>[4x]SNAGGRAAGTGGGGPSAPVDKEVDYAQYFCTYSFLYHQKDMLSDRVRMDAYFNAVFQNKHHFEGKTVLDVGTGSGILAIWSAQAGARKVYAVEATKMADHARALVKANNLDHIVEVIEGSVEDISLPE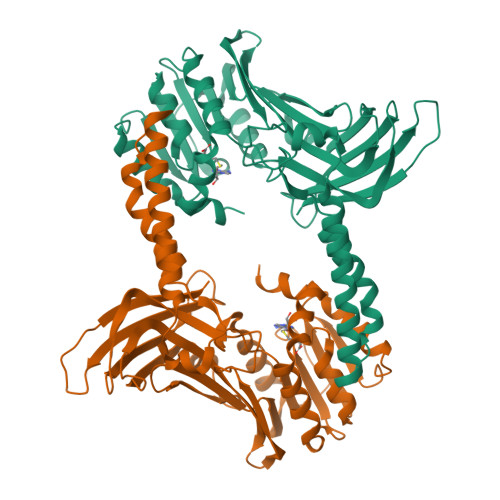KVDVIISEWMGYFLLRESMFDSVISARDRWLKPTGVMYPSHARMWLAPIKSNIADRKRNDFDGAMADWHNFSDEIKSYYGVDMGVLTKPFAEEQEKYYIQTAMWNDLNPQQIIGTPTIVKEMDCLTASVSEIEEVRSNVTSVINMEHTRLCGFGGWFDVQFSGRKEDPAQQEIELTTAPSEQHCTHWGQQVFIMSNPINVEEGDNLNLGLLMSRSKENHRLMEIELNCEIKEASGNPKESFKKTYFIE> GMSAQAKNKLEALKAMTTVVADTGDIEAIKQFKPVDATTNPSLILKAAKLANYQHLIEEAIDWALQIKGNDKNSQTTLENVGDKLAVNIGCEVLTSIPGVISTEVDARLSFDTQATVAKARKLIRLYQDAGIDSDRILIK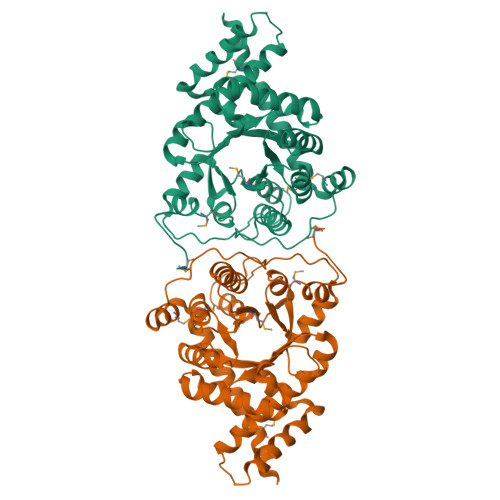IASTWEGIQAAKILEAEGIHCNLTLLFHFAQAQACAEAGTTLISPFVGRILDWYKANSGQSEYSASEDPGVVSVTEIYNFYKSHGFKTIVMGASFRNTGEIEELAGCDRLTISPELLAQLEADTSPLEQKLFPIKETKDTPELLTEASFRWAMNNDPMAHDKLADGIRRFAADQVTLESMLSKKISQRS>MNNLTSIDLSPQTLMAMHISISSQALLNQSYSNLLLSQQLLTSQSMDPGLTVKIKAYQNQLRQQAQVFKQNTVAELIGLYTKASNFAALVNAVNALYSTEDPQVSQK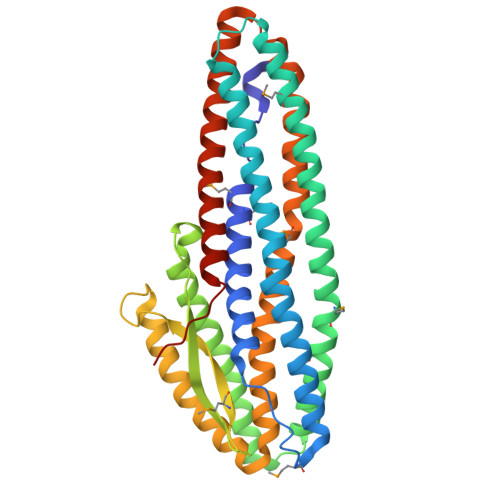GAEMVAALSDVAQHYQAAAQAVHTQLQAKREMLEPLMGNFLNVIDAIEQGLNAEAKQQAQTIAELNEAIAKNIQSIADAGFKAGEGVVQLGQSIVAAVPLGPTDKKPKEAPTAPPKPLSDQASYMISGIQAISAGASGAQQAVNELKANYAKLAVAYRALATANALLSVAKSVQAQAQLFVDTYVLTEQRMALLPTEWGKVAEAYLTAAPIINQAGSAAEIKQAKQIISLNAEKWQLFSKSIDNAKANYAGNNILPEVLEHHHHHH[8x]>MSLFKIRMPETVAEGTRLALRAFSLVVAVDERGGIGDGRSIPWNVPEDMKFFRDVTTKLRGKNVK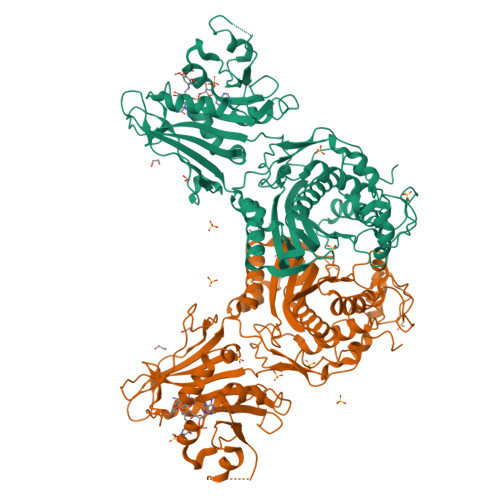PSPAKRNAVVMGRKTWDSIPPKFRPLPGRLNVVLSSTLTTQHLLDGLPDEEKRNLHADSIVAVNGGLEQALQLLASPNYTPSIETVYCIGGGSVYAEALRPPCVHLLQAIYRTTIRASESSCSVFFRVPESGTEAAAGIEWQRETISEELTSANGNETKYYFEKLIPRNREEEQYLSLVDRIIREGNVKHDRTGVGTLSIFGAQMRFSLRNNRLPLLTTKRVFWRGVCEELLWFLRGETYAKKLSDKGVHIWDDNGSRAFLDSRGLTEYEEMDLGPVYGFQWRHFGAAYTHHDANYDGQGVDQIKAIVETLKTNPDDRRMLFTAWNPSALPRMALPPCHLLAQFYVSNGELSCMLYQRSCDMGLGVPFNIASYALLTILIAKATGLRPGELVHTLGDAHVYSNHVEPCNEQLKRVPRAFPYLVFRREREFLEDYEEGDMEVIDYAPYPPISMKMAV[4x]>[2x]RSLGERTVTELILQHQNPQQLSSNLWAAVRARGCQFLGPAMQEEALKLVLLALEDGSALSRKV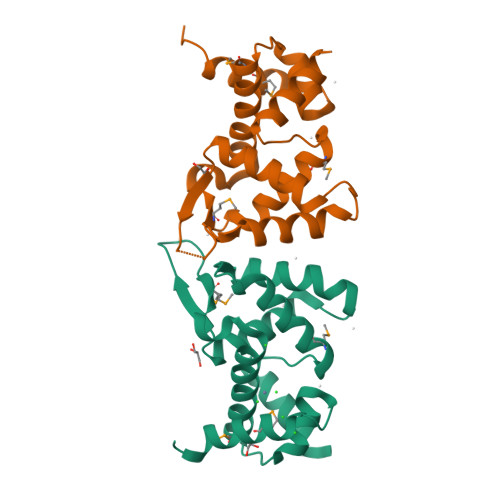LVLFVVQRLEPRFPQASKTSIGHVVQLLYRASCFKVTKRDEDSSLMQLKEEFRTYEALRREHDSQIVQIAMEAGLRIAPDQWSSLLYGDQSHKSHMQSIIDKLQTPA> ACAAACGGCGGATTGACCGTAATGGTAACCGTAGAGGCGACCACCACC;> TTTTTCGGATTCTCGACCGTATCGGCTTTTT;> TTGACCCCCAGAGCCACGCCACCCTCAGAACCTTTGCTTTTT;> ACTCATCTAAAGTACAGACTCCTCAAGAGAAG;> ACTAAAACATCCGCGATACGTTGGACGGAGATTTGTATCACGCGAAAC;> AAGAATACTAAAGACTGAACTGACGACCTTCAAAATGCAA;> ACGAAGGCACGGGTAAAAATGTGAGGATATTCAGGTCTTT;> TTTTTCTCAGATGCCACTAGGTTGAGGCCATCTTTTCATAAT;> TTTTTATACCAAGTCGTTTTTTTTTTCCTGATAAATT;> TGTAGATGGGCGCATCGGATAGGTCCTGCTCCATGTTACT;> AATGCTACTACTATTAGTAGAATTGATGCCACCTTTTCAGCTCGCGCCCCAAATGAAAATATAGCTAAACAGGTTATTGACCATTTGCGAAATGTATCTAATGGTCAAACTAAATCTACTCGTTCGCAGAATTGGGAATCAACTGTTACATGGAATGAAACTTCCAGACACCGTACTTTAGTTGCATATTTAAAACATGTTGAGCTACAGCACCAGATTCAGCAATTAAGCTCTAAGCCATCCGCAAAAATGACCTCTTATCAAAAGGAGCAATTAAAGGTACTCTCTAATCCTGACCTGTTGGAGTTTGCTTCCGGTCTGGTTCGCTTTGAAGCTCGAATTAAAACGCGATATTTGAAGTCTTTCGGGCTTCCTCTTAATCTTTTTGATGCAATCCGCTTTGCTTCTGACTATAATAGTCAGGGTAAAGACCTGATTTTTGATTTATGGTCATTCTCGTTTTCTGAACTGTTTAAAGCATTTGAGGGGGATTCAATGAATATTTATGACGATTCCGCAGTATTGGACGCTATCCAGTCTAAACATTTTACTATTACCCCCT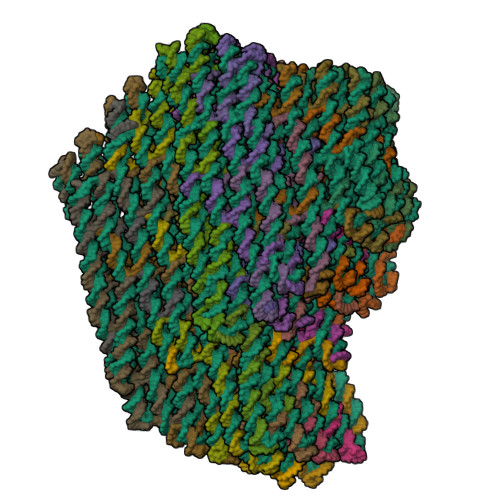CTGGCAAAACTTCTTTTGCAAAAGCCTCTCGCTATTTTGGTTTTTATCGTCGTCTGGTAAACGAGGGTTATGATAGTGTTGCTCTTACTATGCCTCGTAATTCCTTTTGGCGTTATGTATCTGCATTAGTTGAATGTGGTATTCCTAAATCTCAACTGATGAATCTTTCTACCTGTAATAATGTTGTTCCGTTAGTTCGTTTTATTAACGTAGATTTTTCTTCCCAACGTCCTGACTGGTATAATGAGCCAGTTCTTAAAATCGCATAAGGTAATTCACAATGATTAAAGTTGAAATTAAACCATCTCAAGCCCAATTTACTACTCGTTCTGGTGTTCTCGTCAGGGCAAGCCTTATTCACTGAATGAGCAGCTTTGTTACGTTGATTTGGGTAATGAATATCCGGTTCTTGTCAAGATTACTCTTGATGAAGGTCAGCCAGCCTATGCGCCTGGTCTGTACACCGTTCATCTGTCCTCTTTCAAAGTTGGTCAGTTCGGTTCCCTTATGATTGACCGTCTGCGCCTCGTTCCGGCTAAGTAACATGGAGCAGGTCGCGGATTTCGACACAATTTATCAGGCGATGATACAAATCTCCGTTGTACTTTGTTTCGCGCTTGGTATAATCGCTGGGGGTCAAAGATGAGTGTTTTAGTGTATTCTTTCGCCTCTTTCGTTTTAGGTTGGTGCCTTCGTAGTGGCATTACGTATTTTACCCGTTTAATGGAAACTTCCTCATGAAAAAGTCTTTAGTCCTCAAAGCCTCTGTAGCCGTTGCTACCCTCGTTCCGATGCTGTCTTTCGCTGCTGAGGGTGACGATCCCGCAAAAGCGGCCTTTAACTCCCTGCAAGCCTCAGCGACCGAATATATCGGTTATGCGTGGGCGATGGTTGTTGTCATTGTCGGCGCAACTATCGGTATCAAGCTGTTTAAGAAATTCACCTCGAAAGCAAGCTGATAAACCGATACAATTAAAGGCTCCTTTTGGAGCCTTTTTTTTTGGAGATTTTCAACGTGAAAAAATTATTATTCGCAATTCCTTTAGTTGTTCCTTTCTATTCTCACTCCGCTGAAACTGTTGAAAGTTGTTTAGCAAAACCCCATACAGAAAATTCATTTACTAACGTCTGGAAAGACGACAAAACTTTAGATCGTTACGCTAACTATGAGGGTTGTCTGTGGAATGCTACAGGCGTTGTAGTTTGTACTGGTGACGAAACTCAGTGTTACGGTACATGGGTTCCTATTGGGCTTGCTATCCCTGAAAATGAGGGTGGTGGCTCTGAGGGTGGCGGTTCTGAGGGTGGCGGTTCTGAGGGTGGCGGTACTAAACCTCCTGAGTACGGTGATACACCTATTCCGGGCTATACTTATATCAACCCTCTCGACGGCACTTATCCGCCTGGTACTGAGCAAAACCCCGCTAATCCTAATCCTTCTCTTGAGGAGTCTCAGCCTCTTAATACTTTCATGTTTCAGAATAATAGGTTCCGAAATAGGCAGGGGGCATTAACTGTTTATACGGGCACTGTTACTCAAGGCACTGACCCCGTTAAAACTTATTACCAGTACACTCCTGTATCATCAAAAGCCATGTATGACGCTTACTGGAACGGTAAATTCAGAGACTGCGCTTTCCATTCTGGCTTTAATGAAGATCCATTCGTTTGTGAATATCAAGGCCAATCGTCTGACCTGCCTCAACCTCCTGTCAATGCTGGCGGCGGCTCTGGTGGTGGTTCTGGTGGCGGCTCTGAGGGTGGTGGCTCTGAGGGTGGCGGTTCTGAGGGTGGCGGCTCTGAGGGAGGCGGTTCCGGTGGTGGCTCTGGTTCCGGTGATTTTGATTATGAAAAGATGGCAAACGCTAATAAGGGGGCTATGACCGAAAATGCCGATGAAAACGCGCTACAGTCTGACGCTAAAGGCAAACTTGATTCTGTCGCTACTGATTACGGTGCTGCTATCGATGGTTTCATTGGTGACGTTTCCGGCCTTGCTAATGGTAATGGTGCTACTGGTGATTTTGCTGGCTCTAATTCCCAAATGGCTCAAGTCGGTGACGGTGATAATTCACCTTTAATGAATAATTTCCGTCAATATTTACCTTCCCTCCCTCAATCGGTTGAATGTCGCCCTTTTGTCTTTAGCGCTGGTAAACCATATGAATTTTCTATTGATTGTGACAAAATAAACTTATTCCGTGGTGTCTTTGCGTTTCTTTTATATGTTGCCACCTTTATGTATGTATTTTCTACGTTTGCTAACATACTGCGTAATAAGGAGTCTTAATCATGCCAGTTCTTTTGGGTATTCCGTTATTATTGCGTTTCCTCGGTTTCCTTCTGGTAACTTTGTTCGGCTATCTGCTTACTTTTCTTAAAAAGGGCTTCGGTAAGATAGCTATTGCTATTTCATTGTTTCTTGCTCTTATTATTGGGCTTAACTCAATTCTTGTGGGTTATCTCTCTGATATTAGCGCTCAATTACCCTCTGACTTTGTTCAGGGTGTTCAGTTAATTCTCCCGTCTAATGCGCTTCCCTGTTTTTATGTTATTCTCTCTGTAAAGGCTGCTATTTTCATTTTTGACGTTAAACAAAAAATCGTTTCTTATTTGGATTGGGATAAATAATATGGCTGTTTATTTTGTAACTGGCAAATTAGGCTCTGGAAAGACGCTCGTTAGCGTTGGTAAGATTCAGGATAAAATTGTAGCTGGGTGCAAAATAGCAACTAATCTTGATTTAAGGCTTCAAAACCTCCCGCAAGTCGGGAGGTTCGCTAAAACGCCTCGCGTTCTTAGAATACCGGATAAGCCTTCTATATCTGATTTGCTTGCTATTGGGCGCGGTAATGATTCCTACGATGAAAATAAAAACGGCTTGCTTGTTCTCGATGAGTGCGGTACTTGGTTTAATACCCGTTCTTGGAATGATAAGGAAAGACAGCCGATTATTGATTGGTTTCTACATGCTCGTAAATTAGGATGGGATATTATTTTTCTTGTTCAGGACTTATCTATTGTTGATAAACAGGCGCGTTCTGCATTAGCTGAACATGTTGTTTATTGTCGTCGTCTGGACAGAATTACTTTACCTTTTGTCGGTACTTTATATTCTCTTATTACTGGCTCGAAAATGCCTCTGCCTAAATTACATGTTGGCGTTGTTAAATATGGCGATTCTCAATTAAGCCCTACTGTTGAGCGTTGGCTTTATACTGGTAAGAATTTGTATAACGCATATGATACTAAACAGGCTTTTTCTAGTAATTATGATTCCGGTGTTTATTCTTATTTAACGCCTTATTTATCACACGGTCGGTATTTCAAACCATTAAATTTAGGTCAGAAGATGAAATTAACTAAAATATATTTGAAAAAGTTTTCTCGCGTTCTTTGTCTTGCGATTGGATTTGCATCAGCATTTACATATAGTTATATAACCCAACCTAAGCCGGAGGTTAAAAAGGTAGTCTCTCAGACCTATGATTTTGATAAATTCACTATTGACTCTTCTCAGCGTCTTAATCTAAGCTATCGCTATGTTTTCAAGGATTCTAAGGGAAAATTAATTAATAGCGACGATTTACAGAAGCAAGGTTATTCACTCACATATATTGATTTATGTACTGTTTCCATTAAAAAAGGTAATTCAAATGAAATTGTTAAATGTAATTAATTTTGTTTTCTTGATGTTTGTTTCATCATCTTCTTTTGCTCAGGTAATTGAAATGAATAATTCGCCTCTGCGCGATTTTGTAACTTGGTATTCAAAGCAATCAGGCGAATCCGTTATTGTTTCTCCCGATGTAAAAGGTACTGTTACTGTATATTCATCTGACGTTAAACCTGAAAATCTACGCAATTTCTTTATTTCTGTTTTACGTGCTAATAATTTTGATATGGTTGGTTCAATTCCTTCCATAATTCAGAAGTATAATCCAAACAATCAGGATTATATTGATGAATTGCCATCATCTGATAATCAGGAATATGATGATAATTCCGCTCCTTCTGGTGGTTTCTTTGTTCCGCAAAATGATAATGTTACTCAAACTTTTAAAATTAATAACGTTCGGGCAAAGGATTTAATACGAGTTGTCGAATTGTTTGTAAAGTCTAATACTTCTAAATCCTCAAATGTATTATCTATTGACGGCTCTAATCTATTAGTTGTTAGTGCACCTAAAGATATTTTAGATAACCTTCCTCAATTCCTTTCTACTGTTGATTTGCCAACTGACCAGATATTGATTGAGGGTTTGATATTTGAGGTTCAGCAAGGTGATGCTTTAGATTTTTCATTTGCTGCTGGCTCTCAGCGTGGCACTGTTGCAGGCGGTGTTAATACTGACCGCCTCACCTCTGTTTTATCTTCTGCTGGTGGTTCGTTCGGTATTTTTAATGGCGATGTTTTAGGGCTATCAGTTCGCGCATTAAAGACTAATAGCCATTCAAAAATATTGTCTGTGCCACGTATTCTTACGCTTTCAGGTCAGAAGGGTTCTATCTCTGTTGGCCAGAATGTCCCTTTTATTACTGGTCGTGTGACTGGTGAATCTGCCAATGTAAATAATCCATTTCAGACGATTGAGCGTCAAAATGTAGGTATTTCCATGAGCGTTTTTCCTGTTGCAATGGCTGGCGGTAATATTGTTCTGGATATTACCAGCAAGGCCGATAGTTTGAGTTCTTCTACTCAGGCAAGTGATGTTATTACTAATCAAAGAAGTATTGCTACAACGGTTAATTTGCGTGATGGACAGACTCTTTTACTCGGTGGCCTCACTGATTATAAAAACACTTCTCAAGATTCTGGCGTACCGTTCCTGTCTAAAATCCCTTTAATCGGCCTCCTGTTTAGCTCCCGCTCTGATTCCAACGAGGAAAGCACGTTATACGTGCTCGTCAAAGCAACCATAGTACGCGCCCTGTAGCGGCGCATTAAGCGCGGCGGGTGTGGTGGTTACGCGCAGCGTGACCGCTACACTTGCCAGCGCCCTAGCGCCCGCTCCTTTCGCTTTCTTCCCTTCCTTTCTCGCCACGTTCGCCGGCTTTCCCCGTCAAGCTCTAAATCGGGGGCTCCCTTTAGGGTTCCGATTTAGTGCTTTACGGCACCTCGACCCCAAAAAACTTGATTTGGGTGATGGTTCACGTAGTGGGCCATCGCCCTGATAGACGGTTTTTCGCCCTTTGACGTTGGAGTCCACGTTCTTTAATAGTGGACTCTTGTTCCAAACTGGAACAACACTCAACCCTATCTCGGGCTATTCTTTTGATTTATAAGGGATTTTGCCGATTTCGGAACCACCATCAAACAGGATTTTCGCCTGCTGGGGCAAACCAGCGTGGACCGCTTGCTGCAACTCTCTCAGGGCCAGGCGGTGAAGGGCAATCAGCTGTTGCCCGTCTCGCTGGTGAAAAGAAAAACCACCCTGGCGCCCAATACGCAAACCGCCTCTCCCCGCGCGTTGGCCGATTCATTAATGCAGCTGGCACGACAGGTTTCCCGACTGGAAAGCGGGCAGTGAGCGCAACGCAATTAATGTGAGTTAGCTCACTCATTAGGCACCCCAGGCTTTACACTTTATGCTTCCGGCTCGTATGTTGTGTGGAATTGTGAGCGGATAACAATTTCACACAGGAAACAGCTATGACCATGATTACGAATTCGAGCTCGGTACCCGGGGATCCTCTAGAGTCGACCTGCAGGCATGCAAGCTTGGCACTGGCCGTCGTTTTACAACGTCGTGACTGGGAAAACCCTGGCGTTACCCAACTTAATCGCCTTGCAGCACATCCCCCTTTCGCCAGCTGGCGTAATAGCGAAGAGGCCCGCACCGATCGCCCTTCCCAACAGTTGCGCAGCCTGAATGGCGAATGGCGCTTTGCCTGGTTTCCGGCACCAGAAGCGGTGCCGGAAAGCTGGCTGGAGTGCGATCTTCCTGAGGCCGATACGGTCGTCGTCCCCTCAAACTGGCAGATGCACGGTTACGATGCGCCCATCTACACCAACGTAACCTATCCCATTACGGTCAATCCGCCGTTTGTTCCCACGGAGAATCCGACGGGTTGTTACTCGCTCACATTTAATGTTGATGAAAGCTGGCTACAGGAAGGCCAGACGCGAATTATTTTTGATGGCGTTCCTATTGGTTAAAAAATGAGCTGATTTAACAAAAATTTAACGCGAATTTTAACAAAATATTAACGTTTACAATTTAAATATTTGCTTATACAATCTTCCTGTTTTTGGGGCTTTTCTGATTATCAACCGGGGTACATATGATTGACATGCTAGTTTTACGATTACCGTTCATCGATTCTCTTGTTTGCTCCAGACTCTCAGGCAATGACCTGATAGCCTTTGTAGATCTCTCAAAAATAGCTACCCTCTCCGGCATTAATTTATCAGCTAGAACGGTTGAATATCATATTGATGGTGATTTGACTGTCTCCGGCCTTTCTCACCCTTTTGAATCTTTACCTACACATTACTCAGGCATTGCATTTAAAATATATGAGGGTTCTAAAAATTTTTATCCTTGCGTTGAAATAAAGGCTTCTCCCGCAAAAGTATTACAGGGTCATAATGTTTTTGGTACAACCGATTTAGCTTTATGCTCTGAGGCTTTATTGCTTAATTTTGCTAATTCTTTGCCTTGCCTGTATGATTTATTGGATGTT;> TTTTTAAGGTGGCATCAATTCTACAAAGCGGAGACTTCAA;> TTTTTATAAATCACGAGCTTCAAGGATTTTT;> ATATTTTCATTTGGGGAATAACCTCTCCAACATTTTGATA;> TTTTTCGCAAATGGTCCGCGAGCTGCCCGAAATTGCATCATATTATAG;> TTTTTAAATTAAGGATGGCTTATTTCTTTTT;> ATTCTGCGCTGTAGCTTGTCTGGATCAATCATAAATATTT;> TTTTTTAAATCGGTTTGCGGGAGAAGTTTTT;> ATGACCCTGTAATACTTTGTACCACCTCAGAGCATAAAGCTTTTT;> AAGTACGGCAACATGTGTCATTGCTGCCGGAGAGAACTGG;> TTTTTTGCAACTAACATTTTTTTTTTGTTGATTCCCATAGATACA;> TTTTTCCTTTAGAGCTTAAATCGATGGAGGCTTTTT;> ATTGCTGATTTTTGCGCAATAAAGAGGCAAAGAATTAGCATTTTT;> ATCTGGTGAACGAGTAAAAACATTAGTTTCATTCCATGTA;> ATTGCTCCGGTCAGGATAAATTAAAGACAGTCAGCTGCTC;> TTTTTAACGCAAAGCGAAAATACTGCGGAATTTTTT;> CCAGACCGTTTTAATTTACAGGCAGTAGCATTAACATCCATTTTT;> TTAGAGAGTTTTTTTTTTTACCTTTATTTTTTTT;> TTTTTTAAAAATTTTTAGTAATGTGTTAAATTTTTT;> AAAAGATTTTTTTTTTTTAAGAGGAAGAATTTTT;> TTTTTATCATTTTTCATTTTTTTTTTTCAACATT;> TTTTTATTCATTGAATCCAAAGAGGAGTGTCGAA;> GAAAACGACAATCATATAGCCGGAAAAACGAA;> TTTTTCGTCAAGGTAAAGACGAGAACGGCGCATAGCAGCGAA;> ATTCAAAATGCCTGAGAACCCTCATATATTTTTAATAGTA;> GGGTGAGAATATCGCGGAAGCAAAGTTTAGCTGATTTAGTTTGACCAT;> AAGGCCGGAAATGTTTTTAATCATCTCATTATGGGCCTCT;> ATCAATATGATTTTTTTTTTTATTTCCTGTAGTTTTT;> TTTTTTTTTGCAAAAGAAGGAAGAAAGCTTGAGAGCTGCGCAAGCTTGAT;> TAATAGTACTGAGAGTAGAAAGATAAAAGGAATGCTAAAC;> TATTTTTGAGATTTTTTTTTTGATCACCGCCATTTTT;> CAAAAACAGGAAGATTGTATAAGCATGTACCCATAACGCCTCATCAGT;> TTTTTAGCGAAACGGTAAGAGCAACATAACGGAAAAAAAAAG;> AATCAGAAAAGTTTTTTTTTTCCCTAACCAATTTTTT;> GCAGATACCGGTTGATGCTATCAGTTTAAATATTTTT;> TTTTTAGGAAATTGAGAATAGGGGTTTTTTT;> TTTTTCTCGTTTACCAGACGACGACGTAACGAAAATGAAT;> TAAAATTCAAATTGTAAACGTTAATAAAAACCAAAATTTTTT;> GCGTTAAATTTTTGTTCCAGTGCCAACTTTCACCCAATAG;> TTATTTTTTTTTTATAAAACGAACCTATCATAACGTTAGT;> AATCTACGATCGGTTTGCTCCAAATTGATATA;> TTTTTTCAAAAATGGGGGATGAAAGGAACCAGAACCG;> ACCAGAACTCTTAAACATCAGCTTCAGGGTGGAGAGGCGG;> AATAAGGCTTTCAACTAGACTGGAAGAGGGGGAGAGGTCA;> TTTTTCCAGCACCGATATATTCTCCATTTTT;> TGTGAATTGGAAACCAAACAACCAGTTGAGTG;> CAGATGAAAACGGCTAAGACAGCAGGGCGAAA;> CAACTTTGCCCTCAAATGCTTTAAACAGTTCATCAGAAGC;> AGGGAACCTTTTCATGGCTTTTGCACTACGTGTTGTTCCA;> CAGACGGTGAATGACCATAAATCAAAATTTTT;> TCAAGAGTATTCAGTGACAATGACGGCAAAGCGCAACAGC;> AATCTTGATAAAGGCCAGGAAGTTCCGGAACCAGAGCCGC;> CGCTTTTTTTTTTGTTTTCATCGGCATTTTCGGTCATAGC;> TTTTTGATTGGCCTTGATATTCACTGTACTGGTAATATTTTT;> TTTTTGGGGTGCCACCCTCAGCGATTTTTTT;> GTATAAACAGTTAATGCCCCCTGCAGAGCCGCGTCTCTGA;> CAGTGCCCACATGGCTTTTGATGATACAGGAGAAACGAATTTGACAGG;> TTTTTAGTTTTAACGGGGTCAGTGCCTTGAGTAACGCCAGCAGGATCTTC;> TTTTTAACATGAAGATTAGGATTAGCTTTTT;> AGTATTAAGAACCTATTATTCTGATTTTT;> GAGGCTGAATTTACCGTTCCAGTAAAAGCGCACACCAGAA;> AAGGGAAGGTCTGTCCGTTTGGAACGAGACGGGCCATTCG;> GCATCTGCATTAAAGCCAGAATGGAGCGTCAT;> CAGTTTGAGGGGACGACCGTGGGAGCGAGTAACAACCCGTTTTTT;> TTTTTAGGGTAGCCGGTTTTTTTTTTTGTACAGACCA;> CAGAGGCTCTCAGAGCCCACCCTCCTATTTCG;> AATACGTAGAAGATTTTTTTTTTTCGCACGGTCGCT;> TTTTTGCCAGCTTTCCGGTGAGAGAGGCCCGCTTATTACGCA;> TTTTTGGTGAATTGAGTTTTTTTTTTTAGTAAATTGG;> ATCTCCAACAACATTAGGACGTTGGTTTTGCCTAGCGTCC;> TTTTTTCAACCGTACTGAACCCATTACCGAAC;> AATAATAATCGCTATTGTCGTGCCTGATTGCCATCCAGAA;> AACTAAAGAGCGGAGTCAACTAATTCATTTTT;> TTTTTTAGTTGGGTAACGCCATGCTGCAACGCTCACT;> ACTGTTGGGCGCGGGGTTTTTCTTCAGGAAAA;> GAAGGGCGCCATTCAGTGGTTTAATTGCCCTG;> ATCGGTGCACCAGTCATTACAGGTCTGGAGCACTAGCATG;> ACGCCAGCCTGGTGCCACCTTATGCGTAACAAAAATCACCACCCTGAC;> TGGCGAAAAATTCGCGAGGAATACCTACAAAG;> TCTAAAGTAACGCCTGTAGCATTCAATATCAAGCCCTAAA;> ATGCCCTCATAGTTAGTATTTTGTCATAGTAATCGTAAAAAACAAGAG;> AAGCTTGCGTCGACTCTAGAGGATAAAAATCTGAACCACC;> TTTTTTTCCCAGTCACGACGAATTCGTAATCATGAACAGTGC;> ACAGTTTCGAATTGCGTGAGATTTCGATTTTAAGGGTAGCCTAGCTGA;> AACTTTTTTTTTACTTTGTCGTTTTTTTTTTTCTTTCCAGACCTTTTT;> CCAGTACAAACTGATAACCTTTTTTTTTTCTCAATCAATA;> TTTCGTCAAGTATAGCCCCTTCTGACATTCTGATTTACAT;> ACCCTCATGAGGTGAGCACGCTGACTAAAATATCTTTAGG;> CACCCTCAGAGCCACCCCACCCTCAAGTAAGCGTATGTTA;> CACAACATAAACGATTATTATTTAGCCAGTTACAAAATAA;> ACCGAGCTCGTTGTAAAACGACGGAAATCAGC;> CGCTTTTTTTTTTTCACAATTCCAAGCCTGGGAATAGCTA;> AGCTGCATACCCAAAAGAGGAAACAATTGAGCACACCCTG;> TTTTTGCCGTCGAGAGGGAGGAGCCTTTTTTTTTTTTTAATTGT;> GGTGTATCCGTTGAAATGGGGTTTTTACGAGG;> CAGGAGGTAGGAAACCGAACTGGCTACCAGCGAGGGAGGG;> GTGTTTTTTTTTTCCTAATGAGTGGCAGGCGATTGGGAAT;> GGACTCCAACCAGTTTTTTTTTTGCGGATTGGGCGCGCTTTCGATTTTT;> AAGAACGTTCAGTGAGACGCTCATGGAAA;> CACTATTAAACCGTCTAGGAGCGGGCGCTAGGGCGCTTTTTT;> TTCACCAGCAAGAGTCACCGATAGCACCCTCAGGCTGGCT;> CTTCACCGGAGATAGGTCGCCCACCAGGGAGTCAAGAACC;> TTGCAGCAGAAGAACTGTAATAACGTGCTTTC;> ACGCTGGTTTGCCCCAAGCTAACTCATACATATCTTACCG;> AAATTTTTTTTTTTCCTGTTTGATGACTGTAGGAATCAAGTTTGCCTT;> AGAGCCACCACCGGAAGATGGCCCGGGATCGTTTGCGCCG;> TTTTTTCAGTACGTCAAATCGGAACGTTTTT;> AACCATCAAACGTGGCGAGAAAGGCCCGCCGCGGCCGATTTACATCGG;> CCCAAATCCAAAATCATCCATTAAACCAACCTACGAGGCG;> AAGTTTTTGAGGCTTGGCATAACCCAAATCAATCTGGCCTCAACCGTT;> TGGGGTCGATCAAAAGTTTGATTACAAACTATGAAATTAT;> AGGTGCCGCCCGATTTAGAGCTTGGTACTATGCTCGTTGG;> TAAAGCACCCCCTTATTAGCGTTTGCAGGTCAGACTTTTT;> TAAATCGGTAGCGTCAGGTGGTTCCACCATTATAGAGCCA;> GAAGGCTTGAGAAACAAGTTGAGTATATGTACTCATATGCGTTATACA;> CAGATATAAAGGTAAACGGGAGCTGTTGTAGCAGCCGGCG;> GGAATCATGGTGAATTCGTATAACATCACTTGAGGGAGCC;> TTTTTGCCGTTTTTATTTAGCATGTATTTTT;> AGAACGGGCCAATAGCATCAAAATCATAGGTCTTGGGTTA;> TTGCTTCTAGCTTAGATTCTAAGACGGGAGGTAAAAGGGC;> TTTTTGAAACCAATTTTTTTTTTTTTACGTAACCTCCGGCTTAGG;> TTTTTCCTTAGATTTTTTTTTTTTTTCAGGTTTA;> ATAGCGATGTAAATCGCAGTAACATTTAACAAGCGCGTAACCACCACA;> AGTCAATAGAATACCAATAACGGAAAACAAACCGCCGCTACAGGGCGC;> ACGGGGAAAATACTTCAATAGCCCCCTGGCCCCACCGCTT;> TTTTTGGCAAGTGTAGCGACGCCAGAACGTCAGA;> GTTGCTTTTTACCTGAGCAAAAGAGAATTATTTCATTCCA;> GACGAGCAGCAGCACCAACCCTAAACCAGTAGCGAAATCG;> GTAATCAGAATGAAACCGAGAACAAGCAATTTTT;> ATCTTGAGAAGTTTTTTTTTTTGTTTTTATAA;> AAAGGGATGACATTCACCGCCAGCAACGGAATTAATGAAT;> GCCACCGAGGAACGGTGTCACGCTTTTCATTTGAATTTTT;> GTAAAAGAAAAGCGAAATCAGGGCCCGCCTCCTTGAGGAC;> ATCACGCACAATATTAACCGATTGCTAAAGACTTTGAAGC;> AATTAACCAAACAGGAGCTTAATGATCAAGAAAACAAAAT;> CCATTAGCAAGGCTTTTTTTTTTCGGAAACGTCACCTAGCGACA;> TACCTACATTTTGTGGCAGATTCACCAGTCACTTTTT;> ACGCTCAACGTTTTAGTGAATATATCGCTATTCCTTTTTT;> TATTGACGCGGCCTTGGACTCCTTTCCAGTCGGCCACCCT;> ATCACCGTGCAAAATCAGAAAATACACATTAAGAAGCATAAAGTGTAA;> CACCGACTAAAGACACACCAACGCTAACGTTTTT;> GAAAATTCTAACCCACGAACAAAGATAAAACATTTCAGGG;> AATCAATATTGCACCCGATTATACTTCTGAATACCACCAG;> TTTGTCACTCATTAAATACCGCGCTATTAAACTTTCCTTACATTTCAA;> AAGTTTATGCAAACGTCCTGAGTAAGCGGTCCGCAAAATCCCTTATAA;> TTTTTACGACCAGTAATTTGCGTATAAGTTTTTT;> TAAAAGGGACCTGAAAGCGTATTTTT;> AAGGTGGCAACATTTTTTTTTTTATAAAAGAAACGCTGAGCCAT;> AGATAGCCAAGAATTGAGGGAAGCAAGGAGCG;> TTTTTAGAATACGTGGCAAATGCGCG;> CAGAGGGTGCAATAATATTAAAAAGTACCGTAACCTGCAG;> GAAACAATAGCAGCCTTCAGATGACTTTCTTTTT;> TAGTCTTTCAGACAATCGTAAAACAGAAATTTTT;> ATGGCTATACATCGCCAGATAGAACCGGAATACGGCCAAC;> TTAACTGAGCTAATATGAATTGAACTTAAATCAAGATTAG;> CGGGAGAAAGCAGAAGTTACCAGATTAGTACCGGAAACCT;> GCATTAGAAAGGTTATGAGCCAGCAGCAAATGCCCCGGGTATAGCAAG;> GCGGTCAGATAAAAACAGTTAAGCATTGTTTGAGCTACAATTTTATCC;> TATTAACATTTAAGAAAGAACCGCTTGCGTTGGGCGATTATTTTTT;> CAAATAAGACGAGCCGTGTTTCCTGTGTGAAATTGTTATCACAGCCAT;> TTTTGTTTAACGTTTTTTTTTTTCAAAAATGAAAATGAAATAGC;> ACCTTGCTGAACCTCACACAGACAACACTGAGTTTCTGTA;> AAAGCATCATCAACAGTAGAAAGGGACTTTACTTTGCGGAACAAAGAA;> CAACTAATTCCCAATCCCGCCTGCGTCATAGC;> ATCCTTTGCCCGATTTTTTTTTTACGTTATTAATTTTAAAAGTT;> ACATTTGAGGATTTAGAAGTATTAAATTGAGG;> TAGATAATGAATTATCATCATATTTAATCCTGCCAATAAT;> TTTTTCAGAGCCTAATTTAGATTAGAGCCGTCAATGCACTAAAGAATAAC;> ATTATCATAAACAATTCGACAACTCGTATTAATCTGGTCA;> TATTAGCAATTTTTGAAATGGATTGCCAACAGCATTGCAA;> CCAACCATATCAAAATTGAGTAACAACAAAGTGTTGGCAA;> TATGGAAGCAGAGAGAATATGGTTATGATTAACTGGTAAT;> TTTTTAGCGTTGGCAATTCATCAATACCTGATTATTACAGAG;> TTTTTTAAAGCGAACCTCCCGACTTGACGCGAGGTCGTCTGATTTAGACA;> AAATTGCGTAGAATCCTTGAAAACAACTTTTTCAAATTTTTT;> ATCCGGTATTAAGACGCTGAGAAGCAAATCCAGCCTGTTT;> TGAGAGACCGGCTGTCCAAGTACCGCACTCATCATCGATA;> TACCTTTTTCATCGTATGAATCTTCACGGAATAAGAGCAAAAGCCCTT;> TTTTTATATTTTAGTTAAGTAGGGCTTTTTT;> TAGATAAGATTGCTTTGTGAATTTAAGCAAATTTGCTATT;> TCCTGAACTATAACTATCGAGCCAGTAATAAGAGAATATAAAGTATTTTT;> AAGAAAAAAAGTAATTAACACCGGTTTTTTTTTTAATCATAATTACTAGA;> ACATGTTCCCGTGTGATAAATAAGGCGTTAAAAAAAGCCT;> TTTTTCCGACAAAAGGTATAATATCCCATCCTAATCAATAAT;> TTTTTTAATTGAGAATCGCCAGCTCAACATTTCATCT;> AACGCCAACATGTAATTTAGGCAGAATAAACAATCAACAAGTTTAGTA;> CCAGTATAAATGGAAACAGTACATTAATTACAGTACCTTT;> AAGCCAACTGGTTTGAAATTCTTATCTGACCT;> AATACCGAAGCTAATGAAATTTAATATTTAACACAAAGAACGCGAGAA;> TAAGAATACTGTCCAGACGACGACAGGCATTTTATGTAAATGCTGATG;> TTTTTTTAAATTAATTTTCTTTTT;> AAATCAATGAATAACCCAGAACGCATCGCAAG;> AAAATCGCGCAGAGGCAGATGATGTTCGCCTGAATCAGAG> SQQDGSLRSRKANLETGAFGKSTRRTRSKAATPAKRED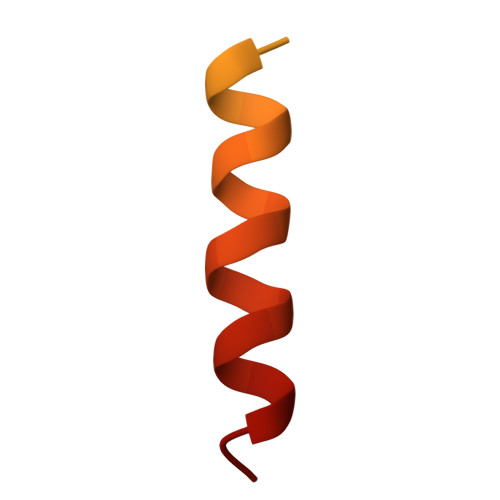PTIAAADKIFSNWLASQ> MSRKRSTKPKPAAKIALKKENDQFLEALKLYEGKQYKKSLKLLDAILKKDGSHVDSLALKGLDLYSVGEKDDAASYVANAIRKIEGASASPICCHVLGIYMRNTKEYKESIKWFTAALNNGSTNKQIYRDLATLQSQIGDFKNALVSRKKYWEAFLGYRANWTSLAVAQDVNGERQQAINTLSQFEKLAEGKISDSEKYEHSECLMYKNDIMYKAASDNQDKLQNVLKHLNDIEPCVFDKFGLLERKATIYMKLGQLKDASIVYRTLIKRNPDNFKYYKLLEVSLGIQGDNKLKKALYGKLEQFY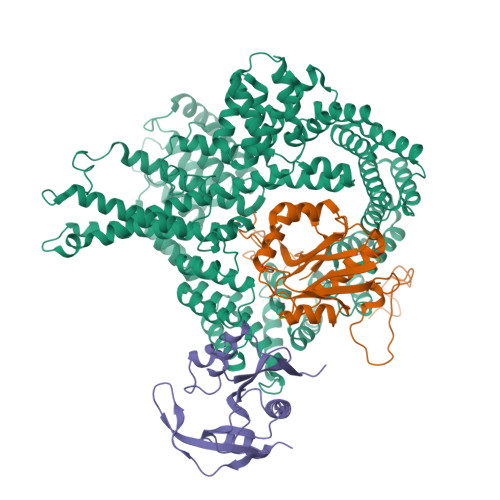PRCEPPKFIPLTFLQDKEELSKKLREYVLPQLERGVPATFSNVKPLYQRRKSKVSPLLEKIVLDYLSGLDPTQDPIPFIWTNYYLSQHFLFLKDFPKAQEYIDAALDHTPTLVEFYILKARILKHLGLMDTAAGILEEGRQLDLQDRFINCKTVKYFLRANNIDKAVEVASLFTKNDDSVNGIKDLHLVEASWFIVEQAEAYYRLYLDRKKKLDDLASLKKEVESDKSEQIANDIKENQWLVRKYKGLALKRFNAIPKFYKQFEDDQLDFHSYCMRKGTPRAYLEMLEWGKALYTKPMYVRAMKEASKLYFQMHDDRLKRKSDSLDENSDEIQNNGQNSSSQKKKAKKEAAAMNKRKETEAKSVAAYPSDQDNDVFGEKLIETSTPMEDFATEFYNNYSMQVREDERDYILDFEFNYRIGKLALCFASLNKFAKRFGTTSGLFGSMAIVLLHATRNDTPFDPILKKVVTKSLEKEYSENFPLNEISNNSFDWLNFYQEKFGKNDINGLLFLYRYRDDVPIGSSNLKEMIISSLSPLEPHSQNEILQYYL;> MPINIRRATINDIICMQNANLHNLPENYMMKYYMYHILSWPEASFVATTTTLDCEDSDEQDENDKLELTLDGTNDGRTIKLDPTYLAPGEKLVGYVLVKMNDDPDQQNEPPNGHITSLSVMRTYRRMGIAENLMRQALFALREVHQAEYVSLHVRQSNRAALHLYRDTLAFEVLSIEKSYYQDGEDAYAMKKVLKLEELQISNFTHRRLKENEEKLEDDLESDLLEDIIKQGVNDIIV;> MGRDICTLDNVYANNLGMLTKLAHVTVPNLYQDAFFSALFAEDSLVAKNKKPSSKKDVHFTQMAYYSEIPVGGLVAKLVPKKQNELSLKGIQIEFLGVLPNYRHKSIGSKLLKFAEDKCSECHQHNVFVYLPAVDDLTKQWFIAHGFEQVGETVNNFIKGVNGDEQDAILLKKHIS>[2x]ETGGNQNQLLSTLATIRTGKKQVSNCSTNIPLVNDLRFINGINKFIIEDYATHDFSIGHPLNMPSFIPTATSPNGCTRIPSFSLGKTHWCYTHNVINANCKDHTSSNQYISMGILVQTASGYPMFKTLKIQYLSDGLNRKSCSIATVPDGCAMYCYVSTQLETDDYAGSSPPTQKLTLLFYNDTVTERTISPTGLEGNWATLVPGVGSGIYFENKLIFPAYGGVLPNSTLGVKSAREFFRPVNPYN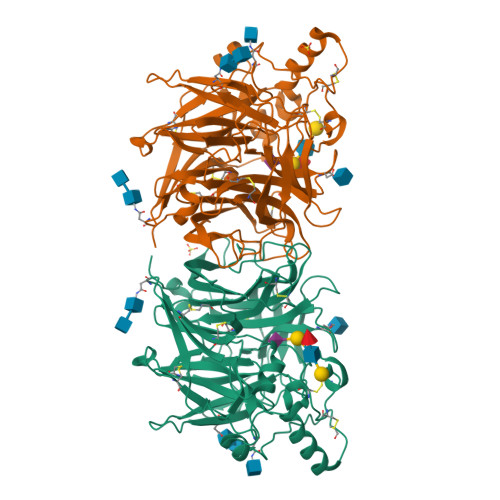PCSGPQQDLDQRALRSYFPSYFSNRRVQSAFLVCAWNQILVTNCELVVPSNNQTLMGAEGRVLLINNRLLYYQRSTSWWPYELLYEISFTFTNSGQSSVNMSWIPIYSFTRPGSGNCSGENVCPTACVSGVYLDPWPLTPYSHQSGINRNFYFTGALLNSSTTRVNPTLYVSALNNLKVLAPYGNQGLFASYTTTTCFQDTGDASVYCVYIMELASNIVGEFQILPVLTRLTITGTKHHHHHH>[4x]PPTNAERLHEFHRAIGAATPERPTPPPPELLRLRQTLLDEESAEVRAEIDHLL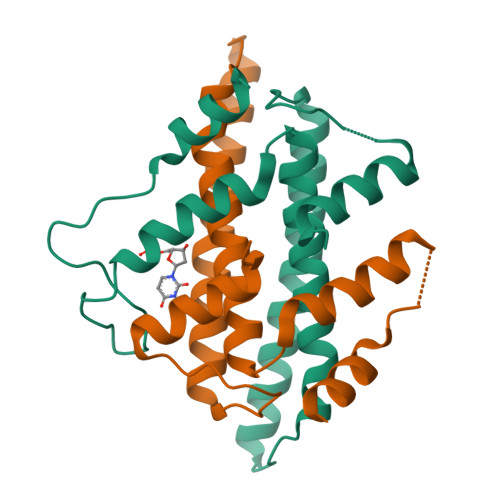ARQAAGEALSAGDLAPLAHALADLLYVTYGALDQLGIDADAVFAEVHRANLSKASGPRRADGKQLKPEGWRPADVRGVIERLQHA>[12x]GSQQFPQFHVKSGLQIKKNAIIDDYKVTSQVLGLGINGKVLQIFNKRTQEKFALKMLQDCPKARRE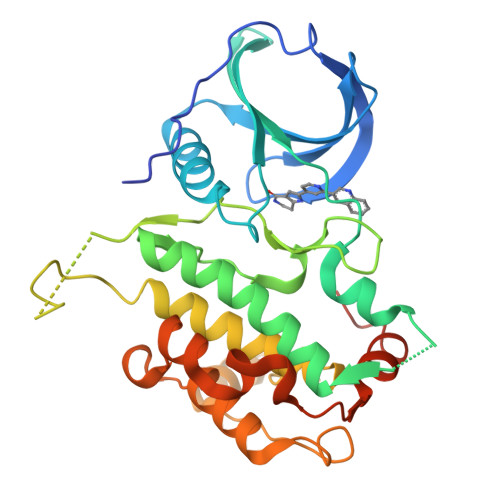VELHWRASQCPHIVRIVDVYENLYAGRKCLLIVMECLDGGELFSRIQDRGDQAFTEREASEIMKSIGEAIQYLHSINIAHRDVKPENLLYTSKRPNAILKLTDFGFAKETTSHNSLTTPCYTPYYVAPEVLGPEKYDKSCDMWSLGVIMYILLCGYPPFYSNHGLAISPGMKTRIRMGQYEFPNPEWSEVSEEVKMLIRNLLKTEPTQRMTITEFMNHPWIMQSTKVPQTPLHTSRVLKEDKERWEDVKEEMTSALATMR>MSESPLRLDRLRDFVSALGELLDRHPDEESVLREGRSLLGELVRHDDWLPEEFAQPDPERYQQYLLHADSRQRFSVVSFVWGPGQTTPVHDHRVWGLIGMLRGAEDAQSFELGAEGLRPIGDPVRLSPGQVEAVSPRIGDIHRVFNASPDQPSISIHVYGANIGAVRRAVYLPDGSEKPFISGYSNQFLPNIWDQSKESAR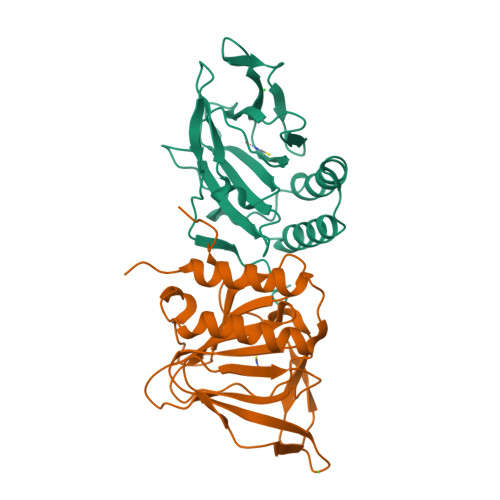PVDLVPR[4x]>[2x]MGSSKPLKGFVICCTSIDLKQRTEISTKATKLGAAYRSDFTKDVTHLIA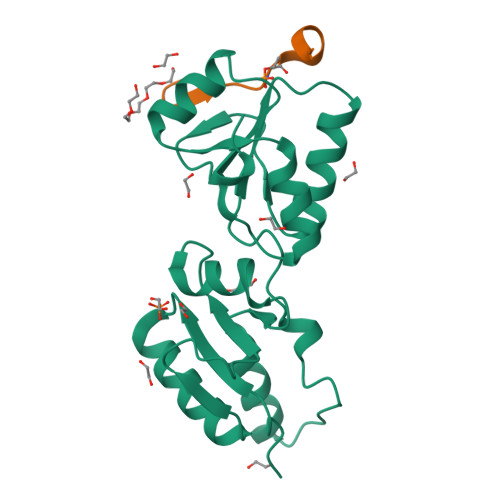GDFDTPKYKFAAKSRPDIKIMSSEWIPVLYESWVQGEDLDDGLLVDKHLLPTLFKCRVCLTNIGQPERSRIENYVLKHGGTFCPDLTRDVTHLIAGTSSGRKYEYALKWKINVVCVEWLWQSIQRNAVLEPQYFQLD;>[2x]GYGRVESTPPAFLP>MAHHHHHHMLKLIVETKTLVQSLGFASSVVEKRNVIPEYANIKLSAKDGNLELSSTNMDLYLSQKIAVQVVSEGECTVSTKTLNDIVRKLPDSELTLTDLGTTGLEIKGKNCKFNLFTLPVSSFPAMDSINPEASFKISCTDFAKIIESTKFSISLDETRYNLNGVYLHIKDKEFCSASTDGHRLSISWVTLEKQIKNFGVILPQKSAEEILKIVKDPKNINEDIEILLSSNKIKFICNENTSMLSKLIDGTFPDYSTFIPESSSSKLVINRKMFADSIERIAIITVEKFRAVKLSLSRETLEISAVGEARGNAKEVINSSQDKESFYEYNSDESLAI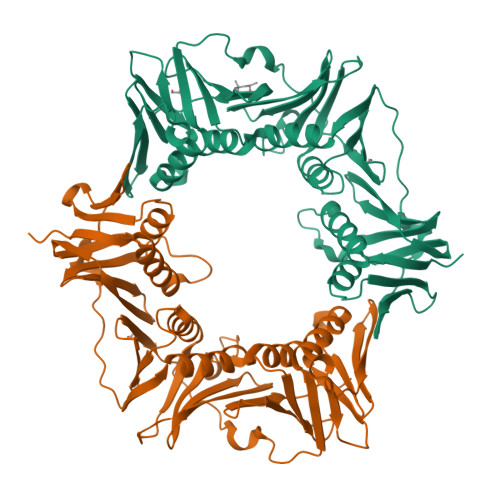GFNPQYLEDVLKAVKSDVVELYFSDVSAPVLIKFPENPKDIFVVMPVKV[2x]>CHREPPPETPDINQLPPSILLKIFSNLSLDERCLSASLVCKYWRDLCLDFQFWKQLDLSSRQQVTDELLEKIASRSQNIIEINISDCRSMSDNGVCVLAFKCPGLLRYTAYRCKQLSDTSIIAVASHCPLLQKVHVGNQDKLTDEGLKQLGSKCRELKDIHFGQCYKISDEGMIVIAKGCLKLQRIYMQENKLVTDQSVKAFAEHCPELQYVGFMGCSVTSKGVIHLTKLRNLSSLDLRHITELDNETVMEIVKRCKNLSSLNLCLNWIINDRCVEVIAKEGQNLKELYLVSCKITDYALIAIGRYSMTIETVDVGWCKEITDQGATLIAQSSKSLRYLGLMRCDKVNEVTVEQLVQQYPHITFSTVLQDCKRTLERAYQMGWTPNMSAASS[2x];>[2x]SVFAYESSVHSTNVLLSLNDQRKKDVLCDVTIFVEGQRFRAHRSVLAACSSYF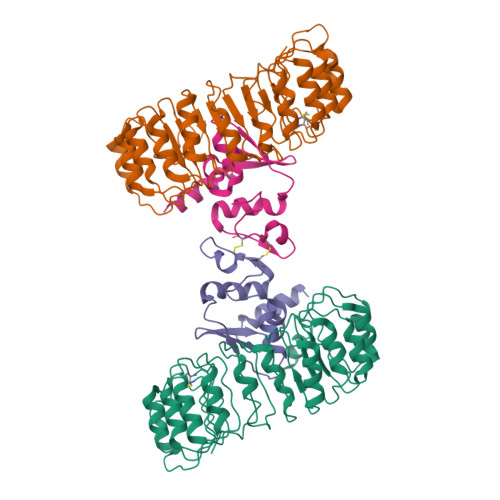HSRIVGQADGELNITLPEEVTVKGFEPLIQFAYTAKLILSKENVDEVCKCVEFLSVHNIEESCFQFLKF> GUGGUCUGAUGAGGCC;> GGCCGAAAC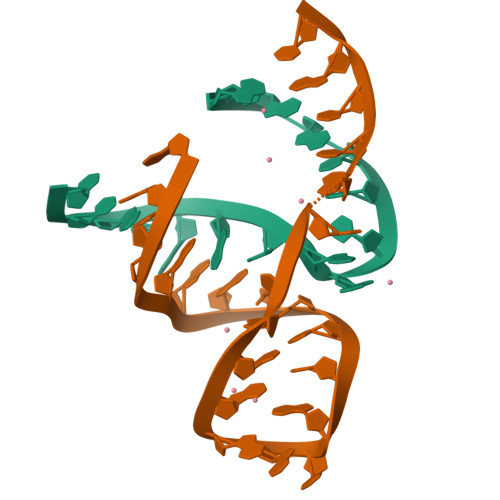UCGUAAGAGUCACCAC> GSWNSGS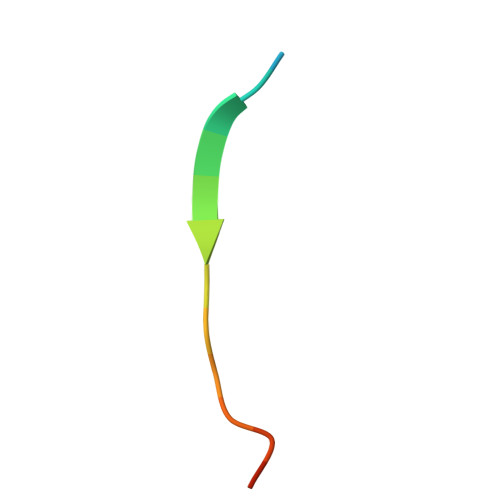SGTGSTGNQ>[2x]MEINVVRETMVRPAG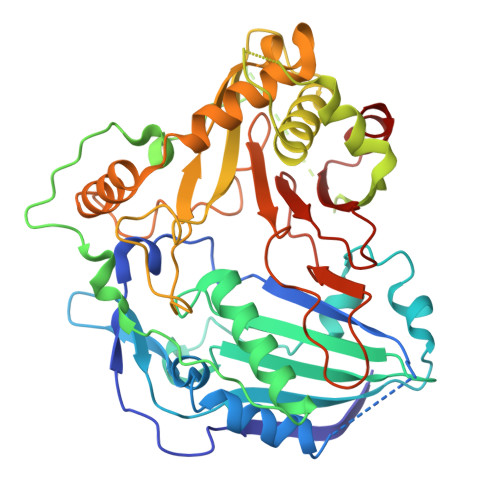ATPQRVLWNSNVDLVIPRIHTASVYFYRPDPSGGEGYFEGGVLREALAKALVPFYPMAGRLKKDENGRFEINCNGEGVLLVEAAAANASVDEYARDFAPDVSFQRLIPSVDYTQDIGSFPLLVLQITRFKCGGASLGVGMEHHVADGMSGITFINTWAAMARGEDPKIVPYIDRTLLRANKPPIPKFPHVEYHPPPLLKHAAATNGHSNGKAKPQAGDDAPPRIAVGLFKFTKEQLQALKSQATDEETNTTYSSYEMLSGHIWRSMCLARGLDDDQETKLYIATDGRARVVPPLPKHYFGNVIFTCTPMALAGDLVSRPLYYAASVIHDAVSRMNDEYLRSALDYLELQPDLYKLVRGAHTFRSPNLGITSWSRLPVYDADFGWGRPVFMGPAVIAFEGLVYVLPSGTGDGSLSISLGLQPEHMPRFEQLIGQI> MKTLVHVASVEKGRSYEDFQKVYNAIALKLREDDEYENYIGYGDDLVRLAWHISGTWDKHDNTGGSYGGTYRFKKEFNDPSNAGLQNGFKFLEPIHKEFPWISSGDLFSLGGVTAVQEMQGPKIPWRCGRVDTPEDTTPDNGRLPDADKDAGYVRTFFQRLNMNDREVVALMGAHALGKTHLKNSGYEGPWGAANNVFTNEFYLNLLNEDWKLEKNDANNE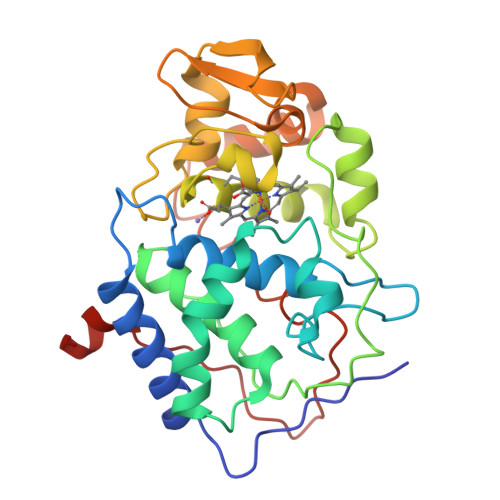QWDSKSGYMMLPTDYSLIQDPKYLSIVKEYANDQDKFFKDFSKAFEKLLENGITFPKDAPSPFIFKTLEEQGL>[4x]HHHHHHGSSELIKENMHMKLYMEGTVNNHHFKCTSEGEGKPYEGTQTMKIKVVEGGPLPFAFDILATSFMYGSKTFINHTQGIPDFFKQSFPEGFTWERITTYEDGGVLTATQD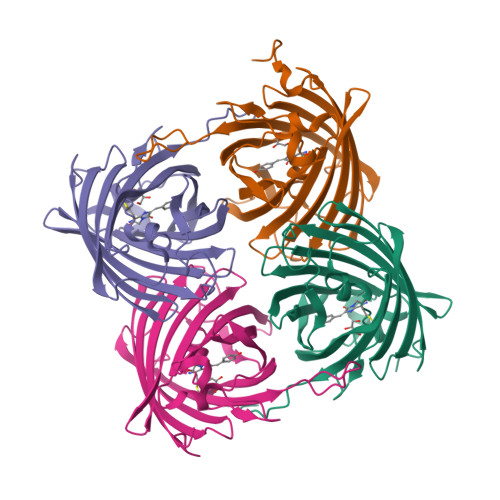TSLQNGCIIYNVKINGVNFPSNGSVMQKKTLGWEANTEMLYPADGGLRGHSQMALKLVGGGYLHCSFKTTYRSKKPAKNLKMPGFHFVDHRLERIKEADKETYVEQHEMAVAKYCDLPSKLGHR> ADEVAILPAPQQLSV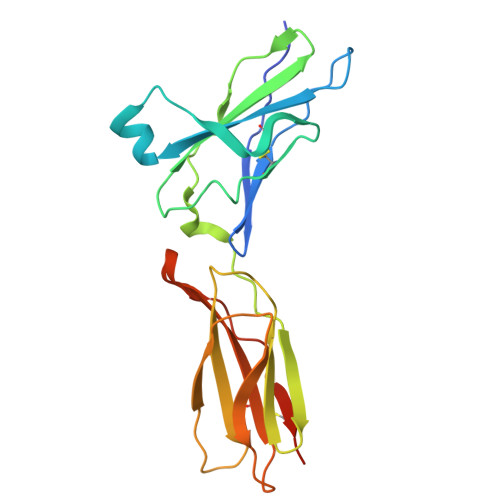LSTNMKHLLMWSPVIAPGETVYYSVEYQGEYESLYTSHIWIPSSWCSLTEGPECDVTDDITATVPYNLRVRATLGSQTSAWSILKHPFNRQSTILTRPGMEITKDGFHLVIELEDLGPQFEFLVAYWRREPGAEEHVKMVRSGGIPVHLETMEPGAAYCVKAQTFVKAIGRYSAFSQTECVEVQGEAIEGR> MAGTSEAVKKWVNKIIEENIIAVFAKTECPYCIKAISILKGYNLNSHMHVENIEKNPDMANIQAYLKELTGKSSVPRIFINKDVVGGCDDLVKENDEGKLKE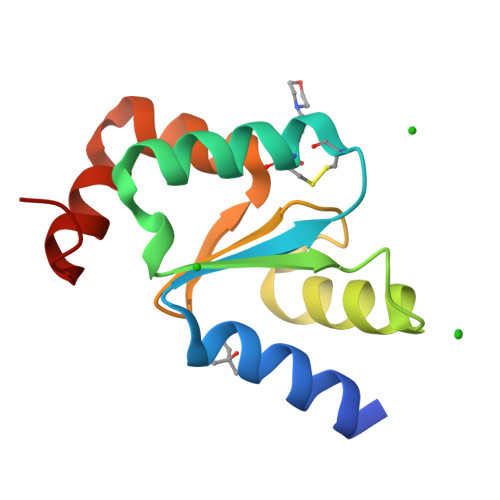RLQKLGLVN>MSRVLLCSAGHSSMVVPEAFHAVPEGFEEVHVFTTDSEKFNPVVLNDFFHSLPNVRFSITKCHGLADILNERDFEFYQEMLWQWYLTKMPDNELPYVCLSGGIKSMSASLQKAATLFGAQSVFHVLADNNPRNIEEMFDALQKGQIHFIEMGYEPGWAALRRLKKI[2x]

In order to identify novel CARF effectors, we used Foldseek18 to search for proteins with structural homology to CARF domain of the Cam1 effector. This method rendered a 600-residue protein containing an N-terminal CARF domain followed by a linker region and a C-terminal adenosine deaminase (ADA) domain, with accession number HAJ98955.1 from an unknown Bacteriodales bacterium (hereafter named CRISPR-associated deaminase, CRISPR-associated adenosine deaminase 1 [Cad1]), for which homologs were already identified in a previous bioinformatic screen. cad1 is located immediately downstream the cas10-csm genes of a type III-A CRISPR locus. Further analysis of cad1 homologs showed that over 70% associate in genomes containing type III systems (mostly belonging to the A and B subtypes) and exist within many unique phyla of bacteria. These data suggest that Cad1 is a widespread effector in type III CRISPR-Cas systems. Altogether, these data demonstrate that Cad1 deaminates ATP molecules to ITP through the formation of an hexameric complex that requires a Mg+2 or Mn+2 cofactor and an activating cA4 or cA6 ligand. While the triggering of a growth arrest in the host is a common strategy of all CARF effectors, we believe that Cad1 introduces a new mode of defense for CRISPR-Cas systems that couples nucleotide deamination activity to a sequence-specific, RNA-guided adaptive immune response.

To further test this finding, we purified a hexa-histidyl-tagged CARF domain (residues 1–185, Cad1-CARF-His6) and tested the binding of different cOAs using isothermal titration calorimetry (ITC). We found that Cad1-CARF-His6 binds to both cA6 and cA4 with a kD of 30 and 700 nM, respectively. We also co-crystallized cA6 and cA4 with Cad1-CARF-His6 and solved the crystal structures at 1.8 and 2.4 Å resolution, respectively. Although both cOA ligands were fully accommodated in the electropositive pocket of apo Cad1-CARF-His6, they affected differently the angle between the two C-terminal legs of the CARF monomers. While cA6 binding produced a minor change (from 58° in the apo structure to 55°), cA4 binding opened this angle to 76°, most likely a consequence of the deep burial of cA4 within the pocket. The Watson-Crick edges of several adenosines of bound cA6 and cA4 form intermolecular hydrogen bonds group of charged residues within the pocket, including K104, that account for the specificity of cOA recognition. Superposition of the structure of this domain within the hexamer with that of the cA4-bound Cad1-CARF-His6 showed good structural correlation (root-mean-square deviation [RMSD] 2.8 Å), with a 3 Å upward shift of the ligand and a decrease in the angle between the C-terminal legs (57°) in the cryo-EM structure. We believe this shift could be due to either the truncation of the full-length Cad1 protein in the case of the crystal structure, crystal-packing forces, or some combination of these factors.>[2x]GSHMRNVAAEQQLRELESTFDGRLGFVALDTATGARIAHRADERFPFCSTFKTMLSAAVLARSAGDAALLQRRIPYAKRDLVRYSPITEKHVGAGMTVAELCAATLQYSDNTAANLLIALLGGPQAVTAYARSIGDATFRLDRRETELNTAIPGDERDTTTIPGDERDTTTPAAMAASVRRLLVGDALGTAQRAQLNAWMLGNKTGDARIRAGVPAGWRVADKTGTGDYGTGNDIGVAYPPDRAPIVF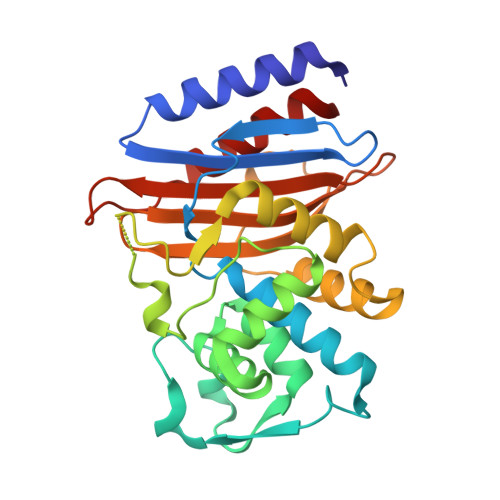VVYTTMRSRNAQARDDVIASAARIAARAFV>[3x]EEGLDFPEYDGVDRVVNVNAKNYKNVFKKYEVLALL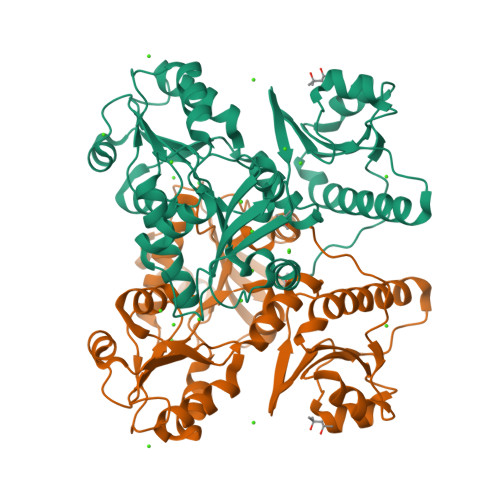YHEPPEDDKASQRQFEMDELILELAAQVLEDKGVGFGMVDSEKDAAVAKKLGLTEEDSVYVFKGDEVIEYDGEFSADTLVEFLLDVLEDPVELIEGERELQAFENIEDDNKLIGYFKNKDSEHYKAYEDAAEEFHPYIPFFATFDSKVAKKLTLKLNEIDFYEAFMEEPVTIPDKPNSEEEIVSFVEAHKRSTLRKLKPESMYETWEDDLDGIHIVAFAEETDPDGYEFLETLKAVAQDNTDNPDLSIIWIDPDDFPLLVPYWEKTFNIDLSAPQIGVVNVTDADSVWMEMDDEEDLPSAEELEDWLEDVLEGEINTEDDDEEDD>MAMPRHGRRPARCSSNRASQWLLLVLGVALAASPRFLLLVEAATYTLTLDKLGPTVNPTTSDAVTFTATVASPDSTTAVFFTLDYGDGVTAETTRTTTGALSTTPTANLVSAGTYTVTYASIGTKFVTLRLYDSAVAPGVLLASKTVPIYVEDSTLTATLLQSGVPRLNLAFSGFKGRVSSSTANRADMWATIQLDTAPGVFESSRIFIGIAPTASTNYDFVIPDQVYNLEGAKTTVLRIYDAPVGGTLLRTFTPAAANAVYVVDPSKYVLTLTVGPTSVTTADQVTFTQTTTEVSYSASATSPILQWRFNWDDPSVVETPLAYPDALTAASNFPTTATAVSSAAASTFRYTSTGSKNARLRLYDGANNVIAEKIVVITVSNAGYTLALAKTTADPVTTDDTIAFSAGAKHLSSTSQVWWTIDYGAGESSPRTALTMTNVGAAAPNAIASLSNQYTSGGTKLATLRIYDRDGVGANTGLLLASTTVTFTVTPVLYALESAVEPFSPIATVAAKWSFRIQRSKATPAGVTESIKCAFFGADTGTAPADLAAWLTAANGAGGLTATILPSSIPSDIISFTRTYAAAAASLQGKLQCFIGSTPLWDPYYPTPVFQVLAAAPTYTLSASVTPAVVPVDTATLWTYNIIRSVPVPAGGPSLPILCSFWDGKTGAAPTTDAGWAALAGSANGKGTSMAPGSTTATCSFTPSYSTTGTATPTLQLIQNSFALDAATTVGFLSPVYTAPAFATVTAASYTISSYLNPVTPVAGGAAAVWRIVITRNAAVTASAKTLTCQMPDNGQGGSPADVTADIAVGGTTTVCVFSIAGYTTATPGPYFATVNVVDGAVTTSHITKNFTVLASGTTAPTYAVTSVVSPATPVKVSTPVTYTFTITRTTAVPAGGIPQPIICEFFNGEGTAPASAAAYWRVSTTIPDADTVVAVMAPGETTTTCTFTTYYTTVSAGGFTAKLMVFGESATAAPLLTSLSVTPSQLLAAVHSFATPMVVAAAVVAVESTTISPNYNPTTPYTNIPTYFTFTLLRDPPVPPSASSGVQFACALYTGQNVNPASAPSAITDAVYKTFTDVTTAVATDANYFADQQLRVVTMAPGTGRVSCTFPTLYAAAGPFSPKFFVFEYASSTVGANALAVADTVTSLTSFTTQAAPTFITGPTNVPQRVPLPKGFRTTCFDGYELIFSNDNYTNGVRVAVDAYPYPVGQCRKCPGGTATMDGYRCIPCPSGYWSNEGARECTACPAGTIAKPAALTARAKYSIDPTTYHFVTHLAMGPESCKKCPKGYFQPNIAGTVCLPCPSGFVSTSGATGCTACSEGTYHTDGVGTTTPGEATSLDTTDTFGSIYPIIPNTCRQCPANTYLPLRGQAAIASMNLAAVSSATPCRPCEDGTWSKAGAAGCQKCPPGTYRNTWFSGQLGSPFITADGVPVATTLTELGSGCSQCPPGTYAPTFGMSVCLPCPAGTFASAPGATACQQCKPGTNSLMGDRTQQMALVVTNAANDFPALRAYTISGMVAGPAYAKPIVTGPDTNFFMAGKSETCSTNLPGYYTDVDGLPIQLPCKPGTFMPFDTATANLLDTGLTVDGTQCYTCQTGTFNDEFSQPVCKACWSGSFASKRGLPTCEIAQPGTFTNVAAAANATFNTATLIPTGLVKGAQAPTPCGMGYFQSSAETTTCTACAVGTYADQAGLAACKPCQPGRYQNSIGQRVCKPCDMGTYSRYGGELCTKCPAGTVASKTGSSQCTPCAAGFYANAPDSATSCRACPRGYYGPYSGAYADNLGDEFEGPRGCYKCPYDFFADRPGVRQCTACPPLDLGGGNLVEQCTEDLGSQRCKPCSLLSKPKTARTEQSPPPPSPSPPPPPPPSPRPPSPNPPSPRPPSPAPPSPNPPPTSPPPSPPPSPPPPRPPPPPPPPPSPPPPNRSPPPPPPASSAINPGGGVNQNGDPVGHRRAILSLMEDEDAEAAQEEQAIVDVDAEMQPQDDE[2x];> MLAILCIAQPAGGQPPSPEPPSPEPPSPAPPSPEPPSPAPPSPEPPSPAPPSPEPPSPAPPSPAPPSPAPPSPPPSPEPPSPAPPSPEPPSPAPPSPEPPSPAPPSPAPPSPAPPSPPPSPEPPSPAPPSPAPPSPAPPSPEPPSPAPPSPAPPSPAPPSPPPSPEPPSPAPPSPEPPSPAPPSPEPPSPAPPSPAPPSPAPPSPPPSPEPPSPEPPSPEPPSPAPQSPEPPSPAPPSPAPPSPSPPSPPPSPEPPSPAPPSPEPPSPAPPSPEPPSPAPPSPAPPSPAPPSPTPPSPEPPSPAPPSPEPPSPAPPSPAPPSPAPPSPEPPSPAPPSPPPSPEPPSPAPPSPEPPSPAPPSPAPPSPAPPSPAPPSPSPPSPPPSPEPPSPEPPSPEPPSPAPPSPAPPSPVPPSPEPPSPEPPSPPPSPAPPSPLPPSPAPPAYSATGIYGDSPWFTTRNGFRWALFKDAATFSAAEEACRDLGGYLANPVSLAVYQDVLDAYSVPFTYLSDTRVWLGISDQDTEGWFYFTSGRGTATVEQVDLITWEDAWDSSHWTQDGSGLDCVAAQLGTATAALTTGAWLEMDCSTPLPFFCSGPTATLTNAPPPGAVAPAPPPPYAAVAYPATSVVVSYATYRLVSPTASTWLAAQQACVGLGGHLASFASAAELTAVRDALVAALAAYSPPYTTSWAPLWIGLYERSLSYGEDWRWSDRSPLTFSGFGQYELNAASNPPTTPNCGALHLDRAGQWSVQGCGTQLQYLCKLANVANAPPPSPPPAAPATARQLAFRFAVGDLTYTLVMQPRSYAAANRYCGSLDPGGTLAVPADAREYMDVMSQVYLYLSSDPAAAGGSALAPPPAASPPPWPPAQVVSALPSQAGEAPFWIGIRWVGAASALGDFTQVDGTSPPTFTQWAAGVYTGPRPVLACASVDPTAGFQYVPAGCGVQLPALCRAATADNAIAPPPSPPSPAPPPPAATAVQTRVGLYLYSLYNEAALTYPEAAAYCRAGGGYLASFHSLAEFNAVWSYMTTTATALAAGDASVWIGYDEIGRNETLLRWLDGGPAAWTHFGLPYTDTEGNDCAAVDQLWGGQWVMDDCLEPRPFICKRLLGISADPAPPPAAVAASPPPLASLPALRNVTVAGVLYQYVASPALSYEAADAACTQYYGVLAWFASASEFNAVMLALQADVAGLYDPSVWFGLYRSYANSADWFWYGNTTLNGTAMADPAQFLFNPTSAACAALGTSLNYQPDNWGGDQRCVAASVLDAGGGSYCYRWDDRACDQRLGFICRVDDRMPLAPSEPQQPPSPPGLPPLPPSPAPPGPDPDPPSPPAPSDPHAPPFPPAPFVPGEPAAPPQKPPTPPPAPPGSDFWSAPWEPPSRPATPDPFPPPPPPPPPPPALPPPGLPPPPPPPPPPPPPPPQHPDLPFAPGEPFYPDPPEAPPPPSFESGVPPPPPPPPPPPPPHAPPLPPSQPGEVSPPPPPPPPPPPGTPTQPSAPLAPAAPGTPTPPAIAESPAVPPPPPPPPPPPPPRTPPLPPKADEHAPPPPPPPPPPPGTPSTPDAPSQPAAPVTQSASPPPALPGAPPPPPPPPPPPPPGMPPTAGAPGAPPPPPPPPPPPGSPDQPSAPAAPSVPAAPQPSPPAEDSTGAVPPPPPPPPPPPPPQTPPAQPSGTTASPPPPPPPPPPPGSPDQPSAPAVPAAPGVPPPPVPAPDTYTAPPPPPPPPPPPPPGTPPSGQPTEPQAPPPPPPPPPPPGTPSAPAAPSQPGVPSVQPDAPPPGLPGAPPPPPPPPPPPPPGVPPTASAPGAPPPPPPPPPPPGAPDQPAAPLAPRPDTQSPGAPPPALPGAPPPPPPPPPPPPPGVPPTAGAPGAPPPPPPPPPPPGSPDQPSAPAAPSVPAAPQPSPPAEDSTGAVPPPPPPPPPPPPPQTPPAPPAGTAASPPPPPPPPPPPGSPDQPSAPATPAAPAVPSPPVPAPDTYTAPPPPPPPPPPPPPGTPPSGQPTEPQAPPPPPPPPPPPGTPSAPAAPSQPSTPAAKVDSPPPGLPDAPPPPPPPPPPPPPGVPPAASAPGAPPPPPPPPPPPGAPDQPATPLAPRPDTQTPGAPPPALPGAPPPPPPPPPPPPPGMPPTAGAPGAPPPPPPPPPPPGSPDQPSAPAAPSVPAAPQPSPPAEDSTGAVPPPPPPPPPPPPPQTPPAQPAGTAASPPPPPPPPPPPGSPDQPSAPATPAAPAVPSPPVPAPDTYTAPPPPPPPPPPPPPGTPPSGQPTEPQAPPPPPPPPPPPGTPSAPAAPSQPSTPAAKVDSPPPGLPDAPPPPPPPPPPPPPGVPPTATAPGAPPPPPPPPPPPGAPDQPAAPARPGPDAPAAPPPAQPGAPPPPPPPPPPPPPSVPPPTPDAAAAPPPPPPPPPPPGSPDQPAHPATPSVPAAPQPPPVDKEDAAPPPPPPPPPPPPPGVPDAPVTTQAPAAPPPPPPPPPPPGTPTMPGAPTKPGAPLAPEQPAEHAPPGAPPPPPPPPPPPPPDAPLPPPARAPDAPPPPPPPPPPPPPPPGAPDAPAAPAQPTASTQPDAPPPALPDAPPPPPPPPPPPPPGTPPAVVAPDAPPPPPPPPPPPGAPDQPAAPARPGPDAPAAPPPAQPGAPPPPPPPPPPPPPSVPPPTPDAAAAPPPPPPPPPPPGSPDQPAHPATPSVPAAPQPPPVDKVDAAPPPPPPPPPPPPPGAPDAPVTTQAPAAPPPPPPPPPPPGTPTMPGAPTKPGAPLAPEQPAEHAPPGAPPPPPPPPPPPPPDASLPPPARAPDAPPPPPPPPPPPGAPDAPAAPAQPTASTQPDAPPPALPDAPPPPPPPPPPPPPGVPPKPAAVDAPPPPPPPPPPPGSPDQPAAPMSPGAPGPTAPPPAHPDAPPPPPPPPPPPPPGVPPPAPGTTPPPPPPPPPPPPPQTPAMPDVPSEGQPAAPIAPSPPVQEDASAPPPPPPPPPPPPPGTPAAPPQVSAPQAPPPPPPPPPPPGTPDAPAMPRLPDAPLTPGAVQQPPAAPGLPPPPPPPPPPPPPQAPPVPGSPNAAPPPPPPPPPPPGAPDQPAAPARPGPDAPSAPPPHLPDAPPPPPPPPPPPPPGVPPPIPDAAAAPPPPPPPPPPPGSPDRPAAPASPDAPGPTAPPPAHPDTPPPPPPPPPPPPPDAPPSPRTHPGKKGDDDAFAPPPPPPPPPPPGMPDMPAVPSQPGAPMPPAAEQVPASPPRLPPPPPPPPPPPPPTTPPPEPDHTAPASPPPPPPPPPPPGTPEMPSVPATPEDVSVLRPDAPPPSLPGAPPPPPPPPPPPPPGAPPALPPQDASPPPPPPPPPPPGTPDAPADIKDWSQPDAPAAPPPALPDAPPPPPPPPPPPPPGVPPPTPVDAPPPPPPPPPPPPPSVPPPPLLDVGVPDLPPSPPPPDQPGAPPPPPPPPPPPPPGVPPPLESPPPDAPPPPPPPPPPPGAPAMPTVPTQPGAPQPPDAADAPAVPPDLPPPPPPPPPPPPPAIPPPTPDAALSPLPPPPPPPPPPPPGTPFTPDTPADWSQPDAPAAPPPGEPNAPPPPPPPPPPPPPGAPPAQPPQDASPPPPPPPPPPPGTPDAPADIKDWSQPDAPATPPPALPDAPPPPPPPPPPPPPGVPPPTPVDAPPPPPPPPPPPPPGAPPPPVLDVGVPDLPPSPPPPDQPGAPPPPPPPPPPPPPGAPPPPNTAPAPPPPPPPPPPPPGTPDMPMVPRAPNAPNVPSPPALPASPPDLPPPPPPPPPPPPPGSPASPIPLAVSPPPPPPPPPPPPPSTPDTPSLPNLPPSSPMPPEIIPPDAPPPPPPPPPPPPPDVPPPGSPPLESPPPPPPPPPPPPATPDAPADIKDWSQPDAPAAPPPAFPDAPPPPPPPPPPPPPGAPPPVPKDSPPPPPPPPPPPPPPGVPPTPEFDPGVPELPPSPPPPDQPSAPPPPPPPPPPPPPGSPPGVPGLPDTPPPPPPPPPPPGTPDMPTLPGAPGPPPPPPPPPPPGAPARDPPPPPPPPPPPPPGMPPGSPSSPLPPPPPPPPPPPPGAPPPPNMPQQPPPLEPDMPPPDFPSTAPPPPPPPPPPPPPGAPPPPSPPPDAPPPPPPPPPPPPEPPPPSLGVPLAPLAPGLPPPPPRPRPPPPKPRPPPPPPPDLPPYAPDPPIPQSPPPPPPPPPPPIPPPPPPPPPPPPPPLAPSPPPPPPPPPEPTAQVDQILGAQPPPPPPLNLTDVSLANITGGRTTTGDAVPDAVTSQPGNTFDVDAYRLVPVVFANVTVVVDAWMQPQLYEKLRRREFADVMRQVLPFSQYLIRVRVNKLTWRIGDYLTEQRNRTLTARGFPPPSPPAPPRAPGSRALSPPPPPPPPPPSNDTSYPRMTLFIQMYAEMTTEADVRAGFGSAALVSSFQFSRFPVYALSLGATSITSYTVYTRRLNVTDNQPPQLTLRGPPEVFVPLYGSYKELGAAAYDLLDGTINDDLVIINLKRWNESEYCCETTFPIDTSQVTEPDKPFIVTYDVFDFVWNSAPTVQRKVHVYDPCAQASNGVERTCPDTRLCSVLGGVCGSATLFSDIRDLATPLTEPDPNNPGITLGIHTLSSDPVYDTIIPNLQLLPLDGLFFVIPPNLDGTPGLQGTLTYLTVGDPWVEPGYIANDDRDDSVQQHVVRRYAELVDTTGPTPPNTPFAITYDVKDVSGNAAITQVRLVFVLCPATLPVLCPPDERVLARPVWYCAAEVCGVPDFFTNALGGAAAVPAVTRNTAPVVRLRDNKYLVTIFDNATYARCPDRGDPTGPCDSGVTATDAEDGDISYKVHAFCADVSTAGVDTMWEAVGLAACQFGNVLKAGRRVITYTVTDTAGATSQISRTLLVMQRCEDGEVQCPDGTCTDFNCFDPSTVITLTLFGNGTDDTTGSGLNVTDGSSFVDSSNFTTSTVNDITGGGSSILTAFASGAPVVSINEPPVIALRNSTLLSQTVQVPQNFVWRNCRASEGPNPATLCELGAQAFDPEEGNLTNTIYVCPPVACLATCSHLNCAGHEFTSKGVRGCVDTGADPGNIFNVIFLVCDNGVPRQSAQVTRTVLIARKCAAGLYECDGVCETVPCAAKAKVARDQVVNNTLPALRLLPPGSSAENAPVSAAGVPLSLTQILTYGVPAPISFSPCASYDANAACAAIAMDVEDGDLTSFINVVDATDCSGKTPNTCLRCRPEQLSLGKCLPGTYRLRYFVEDNSGGISEAFWNFIVESVAVNRVWFLMPPSFNISAPASNSTNATRRFMDQIQVNATRSRGFLVGQLQRFGVDLKDVRSANVSSLALVNTNTDEGQYAINADFCICMINVTLEFTTGLQVNYTVPEVFEIFEPDNFPPPPGRLRPPPVPPSPPPSPAPRPPSPPAPPPPSPGPSPPPAPPDPPSPPPTPPSPPQPPSPPPPPSPAPTPPSPPAPPPVPPSPAPPRPPAPPTPPSPPAPPSPPLPPPSPGPPPGNGNAGRRLIDGTPAVAPAIAPANRVWSWGDDYEMGAVWSPPPPLQRLFNQLRRSMSEPGAAAGAGADVSDYDDDGDGEADWAPVPPADYEEEDPEQDVMVVSAAGTHGPGDSDDNPLPWGLSAAAWGGPAVAGVARKASGAAGGGSGGAQSAPAPAPSVPVPSYLHTALMHASAPSEATGPIDPLLSGAGGPGSAGAGASAAGAPLANTLAAVLGAGEITAASSLSIGARIWQLHVKPALQKQQAAAALAAQAGPHQGLLPVATALYEPFGGFGGGADTGASGLLGAAAAHPAAGSNGAGGGLVGQVVRGDAAKLRASVGVLGKVFTREGEQWDLPGSGALRRAALEEASRAETAAAASDPAASAAASVAAAAIGPRKGQGKGSVGHAATVEAAVAMFSPAALSLVTADSHLDPRTIKGGPVGGLADDFNLHELMGSAKPQPAAKTDDADAGADEPSRRTVVRTLLSEQLVPALAEISRRLEQSQRELDAIRLSPTALGVVEQVGRHGRSRRRLLQTTSGSVANQTASCAPAINATNLATNCTAPPPTTTDMYLAVTLSLIADIDNVNRALSANMTNSTDTISVLDEKFTATDVKYESQYVAYKNLATTYLSALENRTNTVILNLAALAAADATNSMLLSALAGLLKGAVTSAAEEADRLGITTAMLVDGLGLSEENWFFESYQQCLIQRSGSGTTYNFTINREQQAALRYDLETGRVAAPPPPPPARAGFTLLQATQMGRGRSLLGWGSELLSAAAAGAGLGWAGLGPADPQDDSAASAATGSGYHAVRDRRLQTGTVPSTVSAELPQGLTPRLQYGGYELEVAAGRPPAGLTVTYDSRGIPERRRTAGARGNRVVGGLMLHQVRRRLDQVVLGRDSEACQSKFGPLRAECVRSKYSTKNLQDLGGIGEDPVFDRSSSIYSPDVAGRAWAYYNFSEGNSEISTLKLPFGFTHYPVPGLPDGYPVFFDTRLGADRARKLLTYLEDGRYLSPIFSSELRLRLLVYNPDAHVFGYLRAAWDWGGDGVVRLRQWIAAIPATDYGKFISEHQYYMFIPDWIMVLFILLHLASTLLDCVRALQHQRLLQRATEGEPLAGLTADELFRRKRRVKKRYTWRMTPFWVAWEVASCLIQIAALVVLYWFVFVASPGIPTATTYDVYDADVNAPARFFMINKDERGWNPYLASVLQAFQTRSDLKPTNDTIDLAATAAAMAPPSMPPRGGDYRWLLPDDVSGLHALGDMYSYLDNMEYLWNLYFVLQSLVLLMLMVRLMHYVSFQPHLAVIGGAIARAIPMLLYWAVIAGMVVVMLLMLNIIAFGDRLEQLSTISGSAYAVARWLLIKHSDRGNRATITEMLNDNTVILNGGESLVAALVRGLGAIFILFVLYAFVFAILLRQQRMLRRWRHAAPTVGEDLRHMFRWWVQRSWRDAPSNKRLDLTIDWVTRPEVRYTWAYSVLYSAVVRGVAAVAGGTALAKRHPTQHQAVTERAVLLPGGPPGFNSPDEPDPRYCPRYNLRAMMMVFEELLLVNKELRRELFFFMQTNNEDGRTKRMKAMGAPRRAAAAAAVNDASARAMADSLASLLLERFGKRVPRRAARSFDEMMHQLRKRLGTPAGGSGSADGSEFSGSLDGGSARGGDSENSDDDMLPTGVRVGSLKHRGYGVHNQQTVHDLQLQAAVQTAMRNIHTIRENMGRELGDDPQLLATLFVAQFAGQIPEPERRPPGVRPSLYRQRVQQAGSGNSLVNVGAGSAPAPAAPGGPPRPGRSRLGGAAMMGQSPQAAPAPTQGPVAAVLDTNTPEGMLTKALQAMLAPPSTTANAAVSADGTVPAEAEASSASVTDGAPRARPRPKGAKSRARFAADLEIPGNTTSTAGEEAPASPGVASPGAVGSPSGRHNSVSGQLGGSRTARSMLPRHLQPEPRAASFAHPAPATLGSLGQLGSPSSVRSSRSMVMPAGSGSAYFTPSASMGGAAGAATAPGGPTASTGGTDSGAAPQPEPLTIRRPQIHKMRSLGAAAAVAGRMRSFVSGAPGEITPASPTGATSMSAAAAAASLITSPGSYGRSGGSTSMARSGVATPRGDLVSAQISALPLDGTIIFATSAAVVQRLTSHVLQLLRELRGVQADADAMLRSTLVLIERLSAGSVPFPRRAARMVPGVMGSPASSPPVSPQNEKPPGWEDAAVARVAAANAAAAAQRAAVGTASPRLGSSLRVRVEDGAGGAAHGHGAAGANVDDGEDMLPLPPPPALRGVDSYTASPRSLAALQAARGAAGPLSGLLTPPTPTPEASPEKALPPAAAKSAEPAQAEEAPAGESRVVSRAASQAGMKPVDEMREVEPEPELVTFMVQSGMKSRAAGDAAALAAAALAAEEDERREREALAASEGLDSLAPPPGTSSSSGQVHVPAPYGPVEYGAAPHIARLEMAGMRPSSGASQSSDPAIKVLSPASEAHRRASTPKSSHGSRVGSPLLPTEAIRRLSPETSNLSRPGSAAVVDAAPAREAPEEASARRNLPLPSPQGGSRPASVQRDEQGVEVLALPDTVPEGQEAEAGGPMDEPVQGEGEEGEHGALEASRSLGRQPSRIAFSESSMRVRAEDQEEDDELDEPPSATAAAGAGPAQASEPQAPPRAGYIPPPSREPAMQSEPLEGTRPMRPSRSVRLVGVPPPPPPGGVPAPVRRRALASQASLAGTTSQASLGAEASTGEGLVAPPQVLTPEEALSVISQALGTSAPRPIGKPATRHVQLPPDVERRQSQLAKQQELLAAAQAAVAMRRMASNANSRVGSRATSFSAAAAPGAAGLGLQSMDSTGSGAATDAPGGGAGPSTSSAIPPPPGRAAASPLRPGRRALLASAQSGAGFGLDAAPGEEPSNAVQMAAAALERKQAEEAASKAYVDELMNRMRSGMSATGERLALSGRLGSAAGPSGAASPALGAAGGGSRQDSLAGEVSRGSAGLLQQDSLSGTMQLRPSGSIVAPRGAPPMAAFGSLRKPGTGRSSLNLPPMSPLGATPAATGSGEGAGSGLGPIVPPPPLFTNAPGRPQRVSQLMGQGSQGSFGAGSPSAARSAAAQAQLSAFTGDLDVEDFDLDSFGSMRRAPAGPTPKRRQAGDDE

Here, we report the structure of the native C. reinhardtii mastigoneme to ~3.0 Å resolution. Our structure of the C. reinhardtii mastigoneme filament demonstrates that it consists of multiple copies of MST1 around a central single copy of MST3. The structure reveals that MST1 copolymerizes with a second HRGP, MST3, that likely tethers mastigonemes to the membrane through a PKD-like domain. Both proteins exhibit poly(proline) regions that form linear PPII helices, with all proline residues having been converted to O-glycosylated hydroxyprolines.

We traced each mastigoneme filament in cryoSPARC24 and extracted particles along their length with an arbitrary step size. A multi-step processing procedure (Figure S1 and STAR Methods) revealed helical symmetry with a rise of approximately 380 Å and a twist of 172°, creating a filament that is 12 nm at its widest and 6 nm at its thinnest. By exploiting D1 symmetry and using masked local refinement,25 we were able to improve the resolution of the mastigoneme to between 3.0 and 3.1 Å. Residues 43–1,175, which are predicted to be rich in β-strands, form nine consecutive immunoglobulin (Ig)-like domains (D1–D9). Residues 1,176–1,853, rich in cysteine residues, form a single 26-nm domain belonging to the growth factor receptor cysteine-rich domain family with 26 disulfide bonds. Residues 1,854–1,932 form a single, 22-nm long, linear PPII helix, as described in detail later. The mastigoneme filament can be characterized as a double helix with two non-polar MST1 polymer strands that intertwine in a spiral pattern. The fundamental repeat unit within each strand is an antiparallel homodimer formed through an extensive interaction between central cysteine-rich domains. Based on the appearance of the electron cryomicroscopy (cryo-EM) density, all proline residues within the PPII helix are glycosylated. The most likely interpretation is that each serine is O-glycosylated with a single galactose moiety, which is a plant- and algal-specific post-translational modification found on members of the HRGP family. Our analysis revealed unassigned density occupying the central shaft that strongly resembles, and can be partially modeled by, a glycosylated PPII helix.>MRGSHHHHHHGSMDKNIIIGAMTALITPFKNGKVDEQSYARLIKRQIENGIDAVVPVGTTGESATLTHEEHRTCIEIAVETCKGTKVKVLAGAGSNATHAAVGLAKFAKEHGADGILSVAPYYNKPTQQGLYEHYKAIAQSVDIPVLLYNVPGRTGCEISTDTIIKLFRDCENIYGVKEASGNIDKCVDLLAHEPRMMLISGEDAINYPILSNGGKG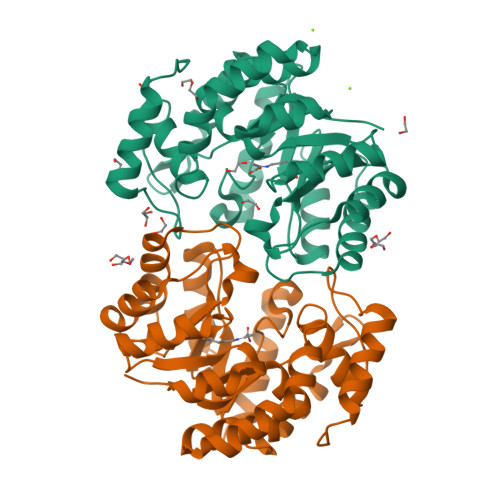VISVTSNLLPDMISALTHFALDENYKEAKKINDELYNINKILFCESNPIPIKTAMYLAGLIESLEFRLPLCSPSKENFAKIEEVMKKYKIKGF[6x]> MVNG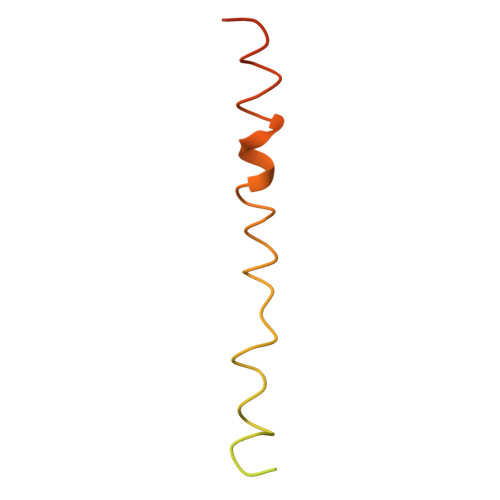DGNPREVIEDLAANNPAIQNIRLRHENKDLKARLENAMEVAGRDFKRAEELEKAKQALEDQRKDLETKLKELQQDYDLAKESTSWDRQRLEKHHHHHH Flavin-dependent halogenases are potentially valuable biocatalysts for the regioselective halogenation of aromatic compounds. Flavin-dependent halogenases require an associated reductase to reduce FAD to FADH2, which is then oxidised by the halogenase and O2 to give C4a-hydroperoxyflavin (FAD-OOH). It is then suggested that chloride attacks the distal oxygen atom of FAD-OOH to generate hypochlorous acid (HOCl),22–24 which H-bonds with an active site lysine residue positioning the electrophile in a spatially defined orientation relative to the aromatic substrate. With PrnA, the carboxylic acid and the amino group of the Trp substrate are engaged in a series of hydrogen bonds to tyrosine (Y443 and Y444), glutamate (E450) and phenylalanine (F454) residues; the indole moiety is stacked between aromatic amino acids (H101, F103 and W455), with an hydrogen bond between the indole NH and a backbone carbonyl group (E346).

In light of this, we sought to engineer PrnA to improve its activity and regioselectivity with anthranilic acid through structure-guided mutagenesis. It seems unlikely that anthranilic acid could contact PrnA active site residues Y443, Y444, E450 and F454, as tryptophan does, while remaining proximal to the catalytic side chains of K79 and E346. Consequently, a series of PrnA mutants were produced with selected active site residues mutated to lysine or arginine. It was reasoned that the additional basic amino acid residues might make contact with the carboxylate group of anthranilic acid to enable tighter substrate binding and effect the orientation of anthranilic acid relative to the catalytic active site residues, thus altering the regioselectivity of halogenation. Mutation of the active site tyrosines (Y443 or Y444) to either lysine or arginine had little effect on the relative activity or regioselectivity with 4. However, the mutation E450K not only increased relative activity ca. 8 fold, but also enhanced ortho selectivity producing 93% 3-chloroanthranilate (4b) compared with 84% observed with the wild-type PrnA (Fig. 3 & Table S1†). Following further mutagenesis PrnA double mutant (E450K/F454K) was found to display a 16-fold increase in activity compared to the wild-type, producing predominantly the para chlorinated product (4a, 54%). In order to rationalise the effects of the selected mutations on the activity of PrnA, X-ray crystal structures for F454K and E450K were determined at 2.4 and 2.3 Å respectively.

> MNKPIKNIVIVGGGTAGWMAASYLVRALQQQANITLIESAAIPRIGVGEATIPSLQKVFFDFLGIPEREWMPQVNGAFKAAIKFVNWRKSPDPSRDDHFYHLFGNVPNCDGVPLTHYWLRKREQGFQQPMEYACYPQPGALDGKLAPCLSDGTRQMSHAWHFDAHLVADFLKRWAVERGVNRVVDEVVDVRLNNRGYISNLLTKEGRTLEADLFIDCSGMRGLLINQALKEPFIDMSDYLLCDSAVASAVPNDDARDGVEPYTSSIAMNSGWTWKIPMLGRFGSGYVFSSHFTSRDQATADFLKLWGLSDNQPLNQIKFRVGRNKRAWVNNCVSIGLSSCFLEPLESTGIYFIYAALYQLVKHFPDTSFDPRLSDAFNAEIVHMFDDCRDFVQAHYFTTSRDDTPFWLANRHDLRLSDAIKEKVQRYKAGLPLTTTSFDDSTYYETFDYKFKNFWLNGNYYCIFAGLGMLPDRSLPLLQHRPESIEKAEAMFASIRREAERLRTSLPTNYDYLRSLRDGDAGLSRGQRGPKLAAQESL6-chloranyl-~{N}-methylsulfonyl-3-(3-naphthalen-1-yloxypropyl)-1~{H}-indole-2-carboxamide | 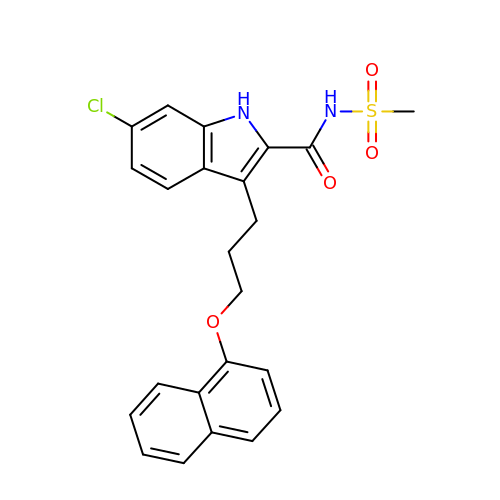C23 H21 Cl N2 O4 S | UTSWEVNFLYKBLS-UHFFFAOYSA-N>GLTPEQKQKKAALSASEGEEVPQDKAPSHVPFLLIGGGTAAFAAARSIRARDPGARVLIVSEDPELPYMRPPLSKELWFSDDPNVTKTLRFKQWNGKERSIYFQPPSFYVSAQDLPHIENGGVAVLTGKKVVQLDVRDNMVKLNDGSQITYEKCLIATGGTPRSLSAIDRAGAEVKSRTTLFRKIGDFRSLEKISREVKSITIIGGGFLGSELACALGRKARALGTEVIQLFPEKGNMGKILPEYLSNWTMEKVRREGVKVMPNAIVQSVGVSSGKLLIKLKDGRKVETDHIVAAVGLEPNVELAKTGGLEIDSDFGGFRVNAELQARSNIWVAGDAACFYDIKLGRRRVEHHDHAVVSGRLAGENMTGAAKPYWHQSMFWSDLGPDVGYEAIGLVDSSLPTVGVFAKATAQDNPKSATEQSGTGIRSESETESEASEITIPPSTPAVPQAPVQGEDYGKGVIFYLRDKVVVGIVLWNIFNRMPIARKIIKDGEQHE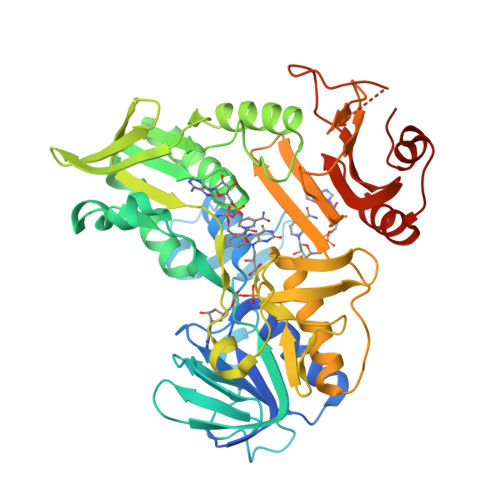DLNEVAKLFNIHED[4x]>GSDRPTPVPLPNSEQFYLENDRGEPYLIQVSWPLHWEDKQTGRGPLPIIYIVDGNALFLTATEAAWRRAAASHFAGGGIIVAIGYPLKGKLYDARRRSFDLTPPTACAPVGYGGADVFLDFIENSVRPAVQARFPQVSLAREALYGHSYGGLLALHALFTRPQSFDCYIASSPSIWWNSLCILHEAKAFVETKKVSHDQSPSLMVSWGSWEQHPPRWADELLDHYEARKRTAAELRMADNALDLCAMLHGCSRLHALIKTEYEGEDHTSVMSCSVSRGL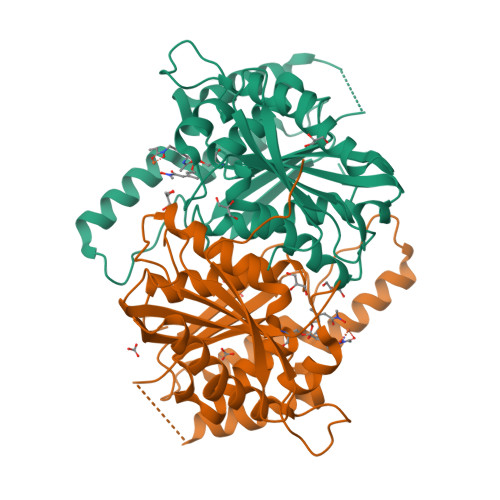TMFFEDWPFHQSG[2x]(3R,5S,9R,26S)-1-[(2R,3S,4R,5R)-5-(6-amino-9H-purin-9-yl)-4-hydroxy-3-(phosphonooxy)tetrahydrofuran-2-yl]-3,5,9-trihydroxy-8,8-dimethyl-10,14,20-trioxo-26-({[(phenylacetyl)amino]acetyl}amino)-2,4,6-trioxa-18-thia-11,15,21-triaza-3,5-diphosphaheptacosan-27-oic acid 3,5-dioxide (non-preferred name) 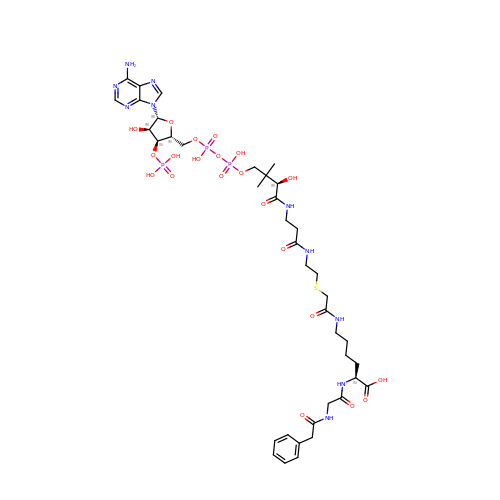| C39 H59 N10 O21 P3 S | UWVFJLUZBIMSSQ-RYFVFCQRSA-N>[4x]APTATLANGDTITGLNAIVNEKFLGIPFAEPPVGTLRFKPPVPYSASLNGQQFTSYG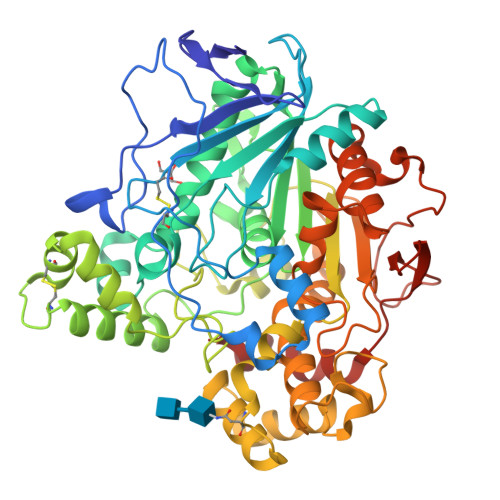PSCMQMNPMGSFEDTLPKNALDLVLQSKIFQVVLPNDEDCLTINVIRPPGTRASAGLPVMLWIFGGGFELGGSSLFPGDQMVAKSVLMGKPVIHVSMNYRVASWGFLAGPDIQNEGSGNAGLHDQRLAMQWVADNIAGFGGDPSKVTIYGESAGSMSTFVHLVWNDGDNTYNGKPLFRAAIMQSGCMVPSDPVDGTYGTEIYNQVVASAGCGSASDKLACLRGLSQDTLYQATSDTPGVLAYPSLRLSYLPRPDGTFITDDMYALVRDGKYAHVPVIIGDQNDEGTLFGLSSLNVTTDAQARAYFKQSFIHASDAEIDTLMAAYTSDITQGSPFDTGIFNAITPQFKRISALLGDLAFTLARRYFLNYYQGGTKYSFLSKQLSGLPVLGTFHGNDIIWQDYLVGSGSVIYNNAFIAFANDLDPNKAGLWTNWPTYTSSSQSGNNLMQINGLGLYTGKDNFRPDAYSALFSNPPSFFV> MHIMEGYLPVTHAIGWSLAAAPFVVAGALKIRKIVAERPEARMTLAAAGAFAFVLSALKIPSVTGSCSHPTGTGLGAVVFGPSVMAVLGVIVLLFQALLLAHGGLTTLGANAFSMAIVGP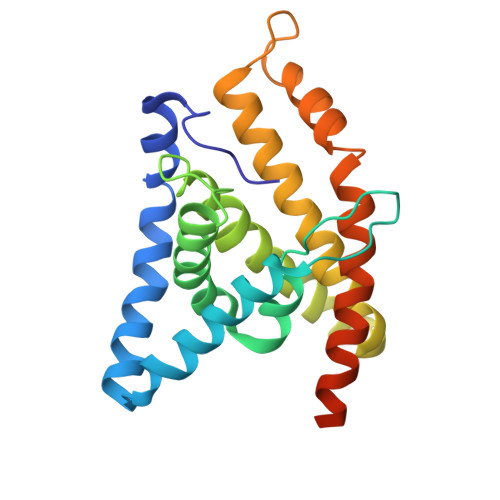WVAFGVYKLAGKAGASMAVAVFLAAFLGDLATYVTTSLQLALAYPDPASGFLGAALKFGSVFALTQIPLAIAEGFLTVIVVDALAGKVADEDKLRILAGEAR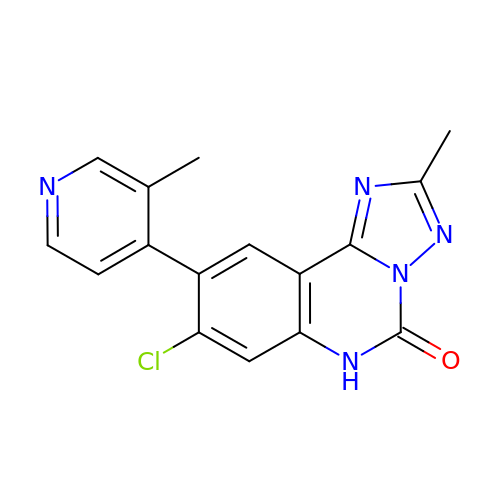(4R,10aP)-8-chloro-2-methyl-9-(3-methylpyridin-4-yl)[1,2,4]triazolo[1,5-c]quinazolin-5(6H)-one | C16 H12 Cl N5 O | FVTXWRGKBOWNPA-UHFFFAOYSA-N> ACC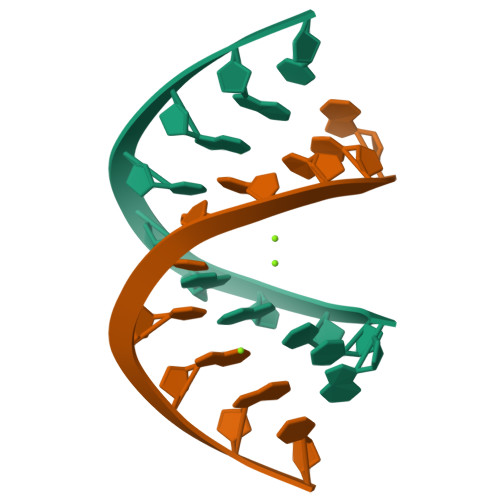GGCCGGT> GPGDPTVFHKRYLKKIRDLGEGHFGKVSLYCYDPTNDGTGEMVAVKALKADAGPQHRSGWKQEIDILRTLYHEHIIKYKGCCEDAGAASLQLVMEYVPLGSLRDYLP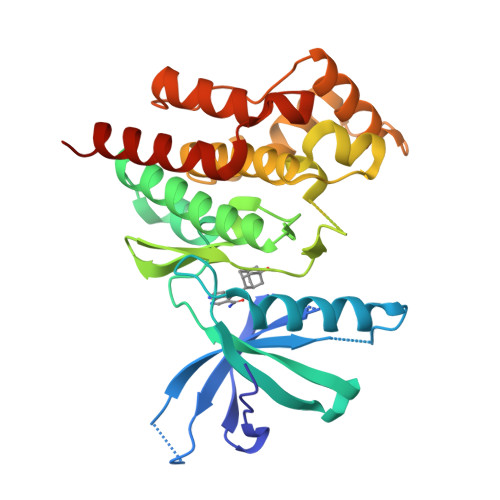RHSIGLAQLLLFAQQICEGMAYLHAQHYIHRNLAARNVLLDNDRLVKIGDFGLAKAVPEGHEYYRVREDGDSPVFWYAPECLKEYKFYYASDVWSFGVTLYELLTHCDSSQSPPTKFLELIGLAQGQMTVLRLTELLERGERLPRPDKCPAEVYHLMKNCWETEASFRPTFENLIPILKTVHEKYQGQAPS>[4x]MAKDIGINSDPNSSSVDKLMKSSGVSNPTYTLVWKVWILAVTLYYAIRIPLTLVFPSLFSPLLPLDILASLALIADIPLDLAFESRRTSGRKPTLLAPSRLPDLLAALPLDLLVFALHLPSPLSLLSLVRLLKLISVQASATRILSYRINPALLRLLSLVGFILLAAHGIACGWMSLQPPSENPAGTRYLSA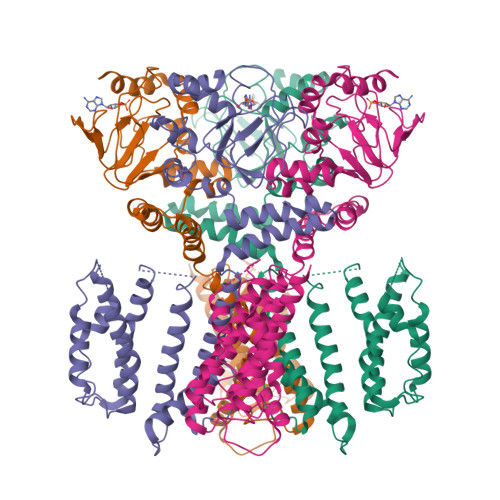FYWTITTLTTIGYGDITPSTPTQTVYTIVIELLGAAMYGLVIGNIASLVSKLDAAKLLHRERVERVTAFLSYKRISPELQRRIIEYFDYLWETRRGYEEREVLKELPHPLRLAVAMEIHGDVIEKVPLFKGAGEEFIRDIILHLEPVIYGPGEYIIRAGEMGSDVYFINRGSVEVLSADEKTRYAILSEGQFFGEMALILRAPRTATVRARAFCDLYRLDKETFDRILSRYPEIAAQIQELAVRRKELESSGLVPRGSVKHHHH> MGSWEIDPKDLTFLKELGTGQFGVVKYGKWRGQYDVAIKMIKEGSMSEDEFIEEAKVMMNLSHEKLVQLYGVCTKQRPIFIITEYMANGCLLNYLREMRHRFQTQQLLEMCKDVCEAMEYLESKQFLHRDLAARNCLVNDQGVVKVSDFGLSRYVLDDEYTSSVGSKFPVRWSPPEVLMYSKFSSKSDIWAFGVLMWEIYSLGKMPYERFTNSETAEHIAQGLRLYRPHLASEKVYTIMYSCWHEKADER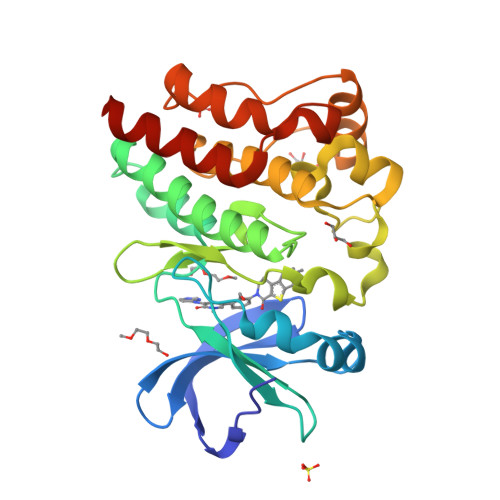PTFKILLSNILDVMDENLYFQ> PQLPEVETIRRTLLPLIVGKTIEDVRIFWPNIIRHPRDSEAFAARMIGQTVRGLERRGKFLKFLLDRDALISHLRAE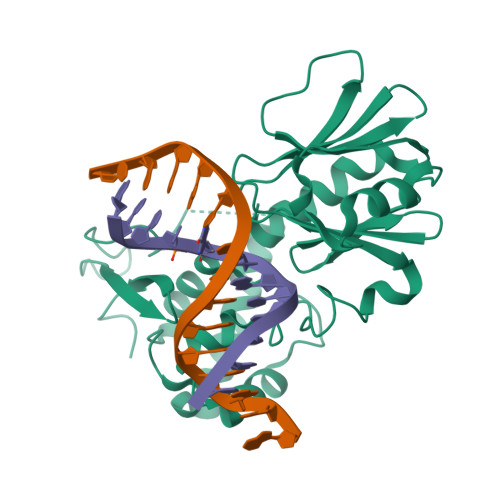GRYAVASALEPLEPHTHVVFCFTDGSELRYRDVRKFGTMHVYAKEEADRRPPLAELGPEPLSPAFSPAVLAERAVKTKRSVKALLLDCTVVAGFGNIYVDESLFRAGILPGRPAASLSSKEIERLHEEMVATIGEAVMKGGSTVRTYVNTQGEAGTFQHHLYVYGRQGNPCKRCGTPIEKTVVAGRGTHYCPRCQR> MSVDRYSGMEGTEHIRFQRLVQVCNKALEESIRKLQSWEKIHECFPNYGQTREGIENLTVCQQQVIKLWSNLSRVEFDAIFHERSIEEKLNQLD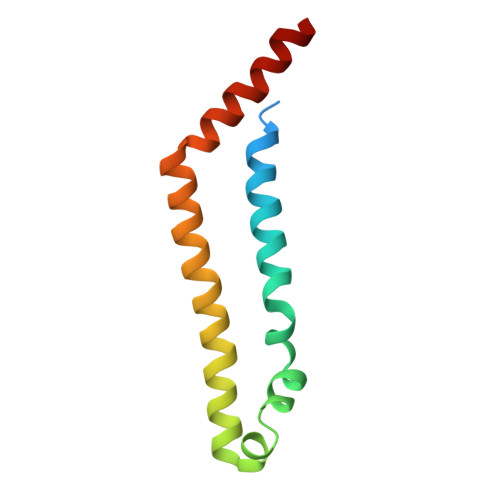DLINKARS>[2x]RRTYTLADYLKNTFRVKSYSLRWVSDSEYLYKQENNILLFNAEHGNSSIFLENSTFEIFGDSISDYSVSPDRLFVLLEYNYVKQWRHSYTASYSIYDLNKRQLITEEKIPNNTQWITWSQEGHKLAYVWKNDIYVKIEPHLPSHRITSTGKENVIFNGINDWVYEEEIFGAYSALWWSPNGTFLAYAQFNDTGVPLIEYSFYSDESLQYPKTVWIPYPKAGA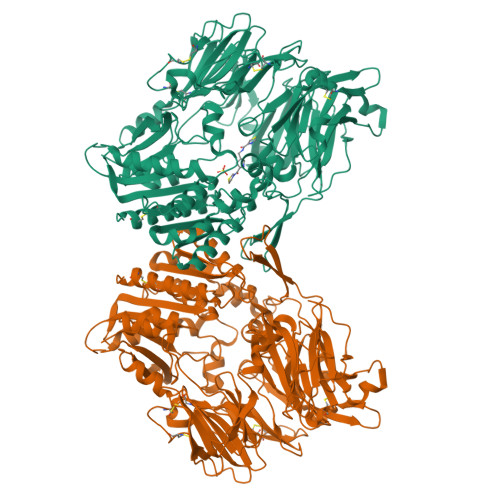VNPTVKFFIVNTDSLSSTTTTIPMQITAPASVTTGDHYLCDVAWVSEDRISLQWLRRIQNYSVMAICDYDKTTLVWNCPTTQEHIETSATGWCGRFRPAEPHFTSDGSSFYKIVSDKDGYKHICQFQKDRKPEQVCTFITKGAWEVISIEALTSDYLYYISNEYKEMPGGRNLYKIQLTDHTNKKCLSCDLNPERCQYYSVSLSKEAKYYQLGCRGPGLPLYTLHRSTDQKELRVLEDNSALDKMLQDVQMPSKKLDFIVLNETRFWYQMILPPHFDKSKKYPLLIDVYAGPCSQKADAAFRLNWATYLASTENIIVASFDGRGSGYQGDKIMHAINKRLGTLEVEDQIEAARQFLKMGFVDSKRVAIWGWSYGGYVTSMVLGSGSGVFKCGIAVAPVSRWEYYDSVYTERYMGLPTPEDNLDHYRNSTVMSRAENFKQVEYLLIHGTADDNVHFQQSAQISKALVDAGVDFQAMWYTDEDHGIASSTAHQHIYSHMSHFLQQCFSLR> AVPE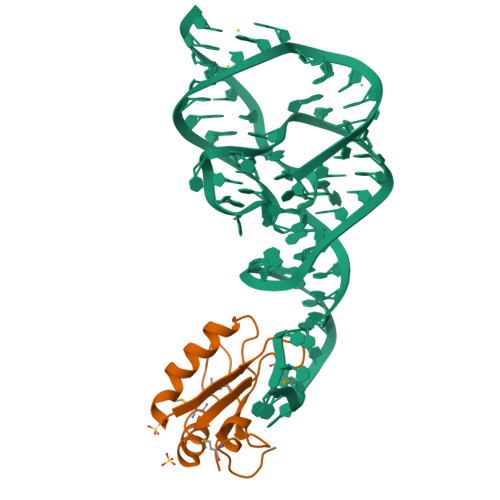TRPNHTIYINNLNEKIKKDELKKSLHAIFSRFGQILDILVSRSLKMRGQAFVIFKEVSSATNALRSMQGFPFYDKPMRIQYAKTDSDIIAKMK>MADNEKLDNQRLKNFKNKGRDLETMRRQRNEVVVELRKNKRDEHLLKRRNVPHEDICEDSDIDGDYRVQNTSLEAIVQNASSDNQGIQLSAVQAARKLLSSDRNPPIDDLIKSGILPILVHCLERDDNPSLQFEAAWALTNIASGTSEQTQAVVQSNAVPLFLRLLHSPHQNVCEQAVWALGNIIGDGPQCRDYVISLGVVKPLLSFISPSIPITFLRNVTWVMVNLCRHKDPPPPMETIQEILPALCVLIHHTDVNILVDTVWALSYLTDAGNEQIQMVIDSGIVPHLVPLLSHQEVKVQTAALRAVGNIVTGTDEQTQVVLNCDALSHFPALLTHPKEKINKEAVWFLS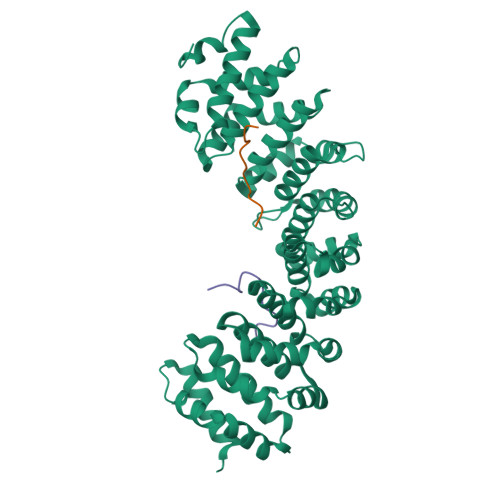NITAGNQQQVQAVIDANLVPMIIHLLDKGDFGTQKEAAWAISNLTISGRKDQVAYLIQQNVIPPFCNLLTVKDAQVVQVVLDGLSNILKMAEDEAETIGNLIEECGGLEKIEQLQNHENEDIYKLAYEIIDQFFSSDDIDEDPSLVPEAIQGGTFGFNSSANVPTEGFQF[2x];>DKEEVQRKRQKLMP[2x];>DRHRIEEKRKRTYETFKSIMKK[2x]>SNSLHWPTSLPSGDAFSSVGTHRFVQKVEEMVQNHMTYSLQDVGGDANWQLVVEEGEMKVYRREVEENGIVLDPLKATHAVKGVTGHEVCNYFWNVDVRNDWETTIENFHVVETLADNAIIIYQTHKRVWPASQRDVLYLSVIRKIPALTENDPETW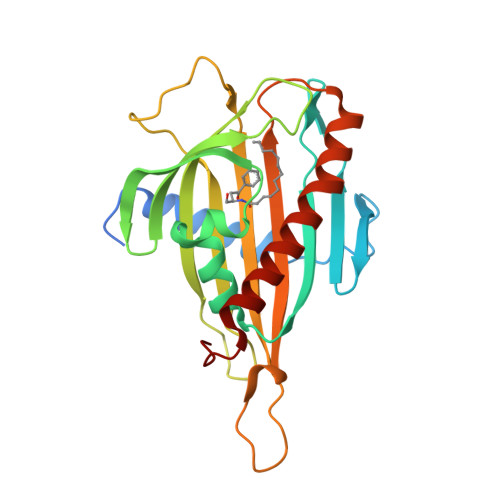IVCNFSVDHDSAPLNNRCVRAKINVAMICQTLVSPPEGNQEISRDNILCKITYVANVNPGGWAPASVLRAVAKREYPKFLKRFTSYVQEKTAGKPILF[2x]> GG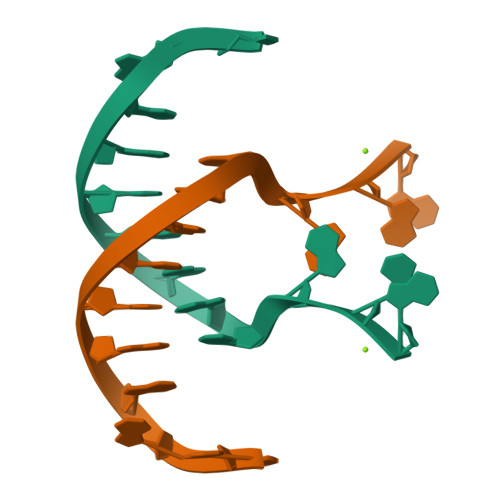ACAGCTGGGAG(6R,7S)-7-({[(cyanomethyl)sulfanyl]acetyl}amino)-7-methoxy-3-{[(1-methyl-1H-tetrazol-5-yl)sulfanyl]methyl}-8-oxo-5-thia-1-azabicyclo[4.2.0]oct-2-ene-2-carboxylic 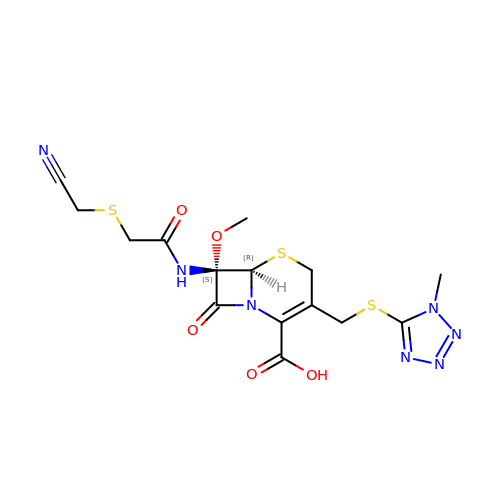acid | C15 H17 N7 O5 S3 | SNBUBQHDYVFSQF-HIFRSBDPSA-N> AMDKSAKAPQITIFDHRGCSRAPKESTGGKAGGQDDEMMVKVASTKVTVSESDAAKKLQEFITFEKGIDGPFTSKN;> AMDKSAKAPVITIFDHRGCSRAPKE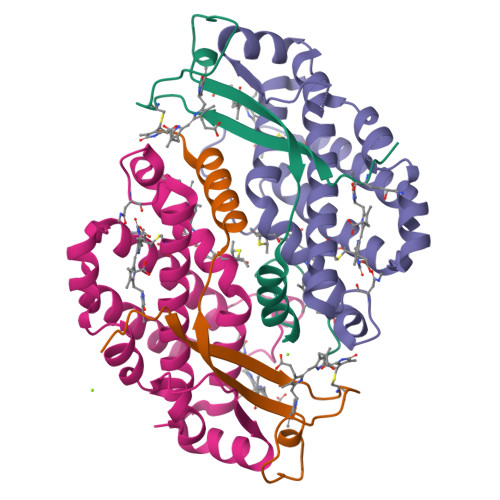YTGAKAGGKDDEMMVKAQSVKIEVSTGTAEGVLATSLAKMTK;>[2x]MLDAFSRVVTNADSKAAYVGGADLQALKKFISEGNKRLDSVNSIVSNASCIVSDAVSGMICENPSLISPSGNCYTNRRMAACLRDGEIILRYVSYALLSGDASVLEDRCLNGLKETYSSLGVPANSNARAVSIMKACAVAFVNNTASQKKLSTPQGDCSGLASEVGGYFDKVTAAIS Bacteriophage E217 infects Pseudomonas aeruginosa and is part of an experimental phage cocktail developed to eradicate P. aeruginosa infections in Galleria mellonella (wax moth) larvae and vertebrate models. E217 is a PB1-like Myoviridae of the Pbunavirus genus characterized by a ~66.2 kbp genome, significantly smaller than the classical enterobacteria phage T4 (~169 kbp). Here, we describe the structure of the whole E217 virion before and after DNA ejection at 3.1 Å and 4.5 Å resolution, respectively, determined using cryogenic electron microscopy (cryo-EM). We identify and build de novo structures for 19 unique E217 gene products, resolve the tail genome-ejection machine in both extended and contracted states, and decipher the complete architecture of the baseplate formed by 66 polypeptide chains.

We determined cryo-EM reconstructions of the extended and contracted E217 sheath at 3.1 Å resolution (FSC = 0.143). Alkalization or spontaneous contraction during purification, observed for ~20% of all virions at neutral pH, triggers tail contraction. This results in sheath compression, with the pitch decreasing to 265 Å and the outer diameter increasing to 250 Å, while the rise and twist decrease to 22.1 Å and 30°, respectively. A secondary structure superimposition of the E217 sheath protein in the extended versus contracted conformations revealed that the N-terminal arms undergo significant movement, with an 80° rotation around residue 24 upon contraction and a maximum displacement of up to 20 Å. Sheath contraction results in a dramatic quaternary structure reorganization with a ~17° clockwise rotation of the β-sheet and extension of the β-strand #4 that becomes nearly straight C-terminal of Gly14. This results in striking compaction and contraction of the sheath that expands in diameter, exposing ~500 Å of the naked tail tube. Upon contraction, tail sheath bodies come into contact laterally, forming a much tighter lattice that releases a large amount of energy. Because of the increased diameter in the contracted state, sheath subunits do not make direct bonds with the tail tube, whose only point of contact is with the gateway C-terminal extension. Sheath subunits make extensive lateral contacts in the contracted state, providing the energetic contribution that makes this conformation thermodynamically stable.

>[13x]MISQSRYIRIISGVGAGAPVAGRKLILRVMTTNNVIPPGIVIEFDNANAVLSYFGAQSEEYQRAAAYFKFISKSVNSPSSISFARWVNTAIAPMVVGDNLPKTIADFAGFSAGVLTIMVGAAEQNITAIDTSAATSMDNVASIIQTEIRKNADPQLAQATVTWNQNTNQFTLVGATIGTGVLAVAKSADPQDMSTALGWSTSNVVNVAGQSADLPDAAVAKSTNVSNNFGSFLFAGAPLDNDQIKAVSAWNAAQNNQFIYTVATSLANLGTLFTLVNGNAGTALNVLSATAANDFVEQCPSEILAATNYDEPGASQNYMYYQFPGRNITVSDDTVANTVDKSRGNYIGVTQANGQQLAFYQRGILCGGPTDAVDMNVYANEIWLKSAIAQALLDLFLNVNAVPASSTGEAMTLAVLQPVLDKATANGTFTYGKEISAVQQQYITQVTGDRRAWRQVQTLGYWINITFSSYTNSNTGLTEWKANYTLIYSKGDAIRFVEGSDVMI5-METHYL-2-[2-OXO-1-(2-THIOPHEN-2-YL-ACETYLAMINO)-ETHYL]-3,6-DIHYDRO-2H-[1,3]THIAZINE-4-CARBOXYLIC 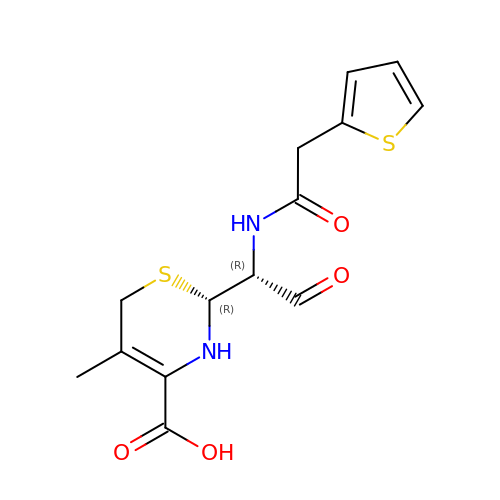ACID | C14 H16 N2 O4 S2 | SFVACKBZMIZHCK-ZWNOBZJWSA-N Like the scCST, the hCST (Ctc1, hStn1 and hTen1) complex is predicted to contain multiple OB-folds and it binds telomeric overhangs with high affinity and some specificity. Overall, hCST plays a role in telomere replication, and may also have a more general role under conditions of replicative stress. To further elucidate the role of hCST at the telomeres, we solved the structures of hTen1 in complex with the N-terminal domain of hStn1 (hStn1N), and the C-terminal domain of hStn1 (hStn1C) alone. These structures reveal that hStn1-Ten1 is a RPA-like complex and a structural homologue of Schizosaccharomyces pombe Stn1Ten1 (spStn1Ten1) and Candida tropicalis Stn1Ten1 (ctStn1Ten1).

To elucidate the function of the human telomeric Stn1-Ten1 complex in telomere biology, we prepared the full-length hStn1-Ten1, the truncated hStn1N-Ten1 and hStn1C proteins to homogeneity. In both RPA and Stn1, the OB fold is a ssDNA-binding domain while the C-terminal domain is important for protein-protein interactions. The additional wHTH motif in hStn1 may allow interaction with a different set of proteins that function at telomeres such as Ctc1.

> AEALSNPGALDLPSLTSLLSEKAKEFLMENRVQSFYQQELEMVESLLSLANQPVIHSASSDQVNFKKDTTSKAIHSIFKNAIQLLQEKGLVFQKDDGFDNLYYVTREDKDLHRKIHRIIQQDCQKPNHMEKGCHFLHILACARLSIRPGLSEAVLQQVLELLEDQSDIVSTMEHYYTAF> ADKELKFLVVDDFSTMRRIVRNLLKELGFNNVEEAEDGVDALNKLQAGGYGFVISCWNMPNMDGLELLKTIRADGAMSALPVLMVIAEAKKENIIAAAQAGASGWVVKPFTAATLEEKLNKI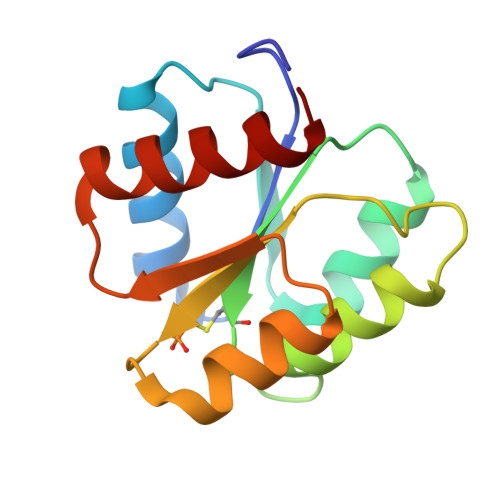FEKLGM N~2~-[2-(5-chloro-1H-pyrrolo[2,3-b]pyridin-3-yl)-5-fluoropyrimidin-4-yl]-N-(2,2,2-trifluoroethyl)-L-alaninamide 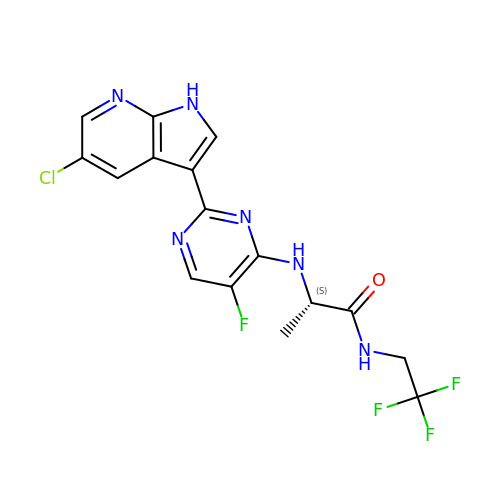| C16 H13 Cl F4 N6 O | JWSTVRZOAIEUAO-ZETCQYMHSA-N> SSTHRKFGGSGGSPFSGSGLSSIAVRSGSYLDAIIIDGVHHGGSGGNLSPTFTFGSGEYISNMTIRSGDYIDNISFETNMGRRFGPYGGSGGSANTLSNVKV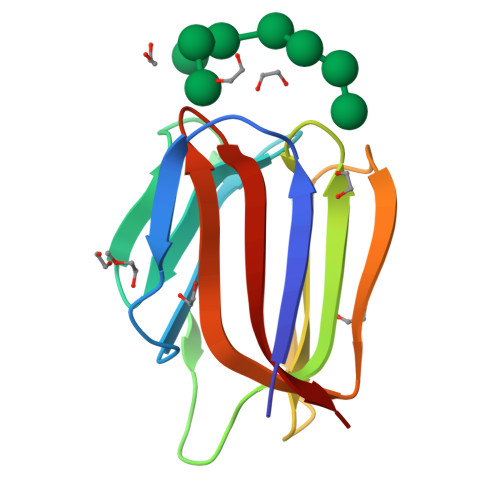IQINGSAGDYLDSLDIYYEQY>MPIDLYYVPGSAPCRNVLLAAKAVGVDLNLKLTDLKSGQHLTPEFIKLNPQHNVPTLDDNGFVLNESRAIMTYLADQYGKDDSLYPKDPKKRAKVNQRLYFDMGTLYQSFGDAYYPHMFGGAPLDEDKKKKLGDALVFLDGFLEKSAFVAGEDLTLADLAIVASISTIEAVEYDLSPYKNINSWYSKVKA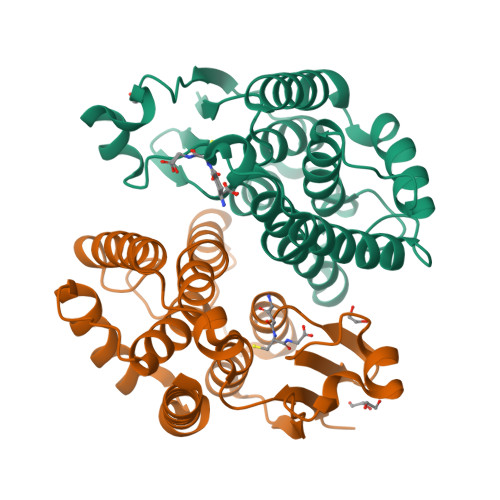AAPGYKEANEEGAKGFGQMFKAMTGK[2x]> WNVRPSDMSNKTFNPIRAIVDNMKVKPNPNKTVISLSIGDPTVFGNLPTDPEVTQAMKDALDSGKYNGYAPSIGYLSSREEVASYYHCPEAPLEAKDVILTSGCSQAIELCLAVLANPGQNILIPRPGFSLYRTLAESMGIEVKLYNLLPEKSWEIDLKQLESLIDEKTACLVVNNPSNPCGSVFSKRHLQKILAVAERQCVPILADEIYGDMVFSDCKYEPMATLSTNVPILSCGGLAKRWLVPGWRLGWILIHDRRDIFGNEIRDGLVKLSQR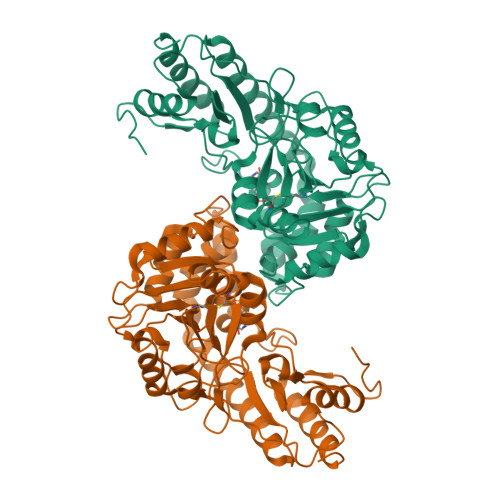ILGPCTIVQGALKSILQRTPQEFYQDTLSFLKSNADLCYGALSAIPGLQPVRPSGAMYLMVGIEMEHFPEFENDVEFTERLIAEQSVHCLPATCFEYPNFFRVVITVPEVMMLEACSRIQEFCEQHY> SLLSNQLHFAKPTARTPLVVLVHGLLGSGADWQPVLSHLARTQCAALTLDLPGHGTNPERHCDNFAEAVEMIEQTVQAHVTSEVPVILVGYSLGGRLIMHGLAQGAFSRLNLRGAIIEGGHFGLQENEEKAARWQHDQQWAQRFSQ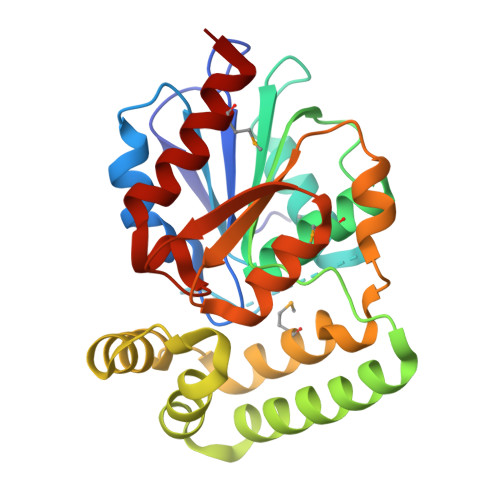QPIEHVLSDWYQQAVFSSLNHEQRQTLIAQRSANLGSSVAHMLLATSLAKQPYLLPALQALKLPIHYVCGEQDSKFQQLAESSGLSYSQVAQAGHNVHHEQPQAFAKIVQAMIHSIID>[2x]STHFDVIVVGAGSMGMAAGYYLAKQGVKTLLVDSFDPPHTNGSHHGDTRIIRHAYGEGREYVPFALRAQELWYELEKETHHKIFTQTGVLVYGPKGGSAFVSETME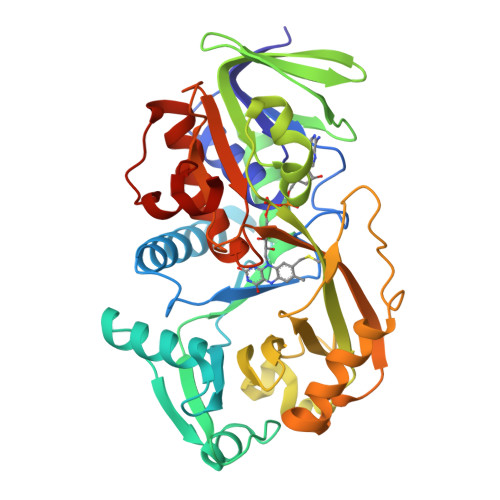AANIHSLEHELFEGKQLTDRWAGVEVPDNYEAIFEPNSGVLFSENCIQAYRELAEAHGATVLTYTPVEDFEVTEDLVTIKTAKGSYTANKLVVSMGAWNSKLLSKLDVEIPLQPYRQVVGFFECDEAKYSNNAHYPAFMVEVENGIYYGFPSFGGSGLKIGYHSYGQQIDPDTINREFGAYPEDEANLRKFLEQYMPGANGELKKGAVCMYTKTPDEHFVIDLHPKYSNVAIAAGFSGHGFKFSSVVGETLAQLATTGKTEHDISIFSLNRDALKKEAVK>[2x]MGHHHHHHMVLMTKPGTSDFVWNGIPLSMELNLWNIKEYSGSVAMKFDGEKITFDADIQNLSPKEPERYVLGYPEFYYGYKPWENHTAEGSKLPVPVSSMKSFSVEVSFDIHHEPSLPLNFAMETWLTREKYQTEASIGDVEIMVWFYFNNLTPGGEKIEEFTIPFVLNGESVEGTWELWLAEWGWDYLAFRLKDPVKKGRVKFDVRHFLDAAGKALSSSARVK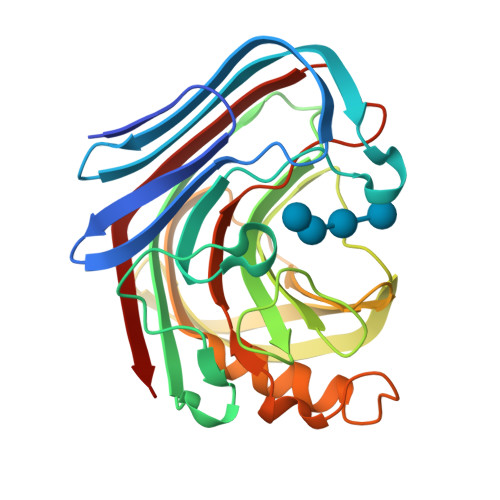DFEDLYFTVWEIGTEFGSPETKSAQFGWKFENFSIDLEVRE>[4x]MGSSHHHHHHSGLVPRGSHMATPPKRSSPSFSASSEGTRIKKISIEGNIAAGKSTFVNILKQLSEDWEVVPEPVARWSNVQSTQDEFEELTMSQKNGGNVLQMMYEKPERWSFTFQTYACLSRIRAQLASLNGKLKDAE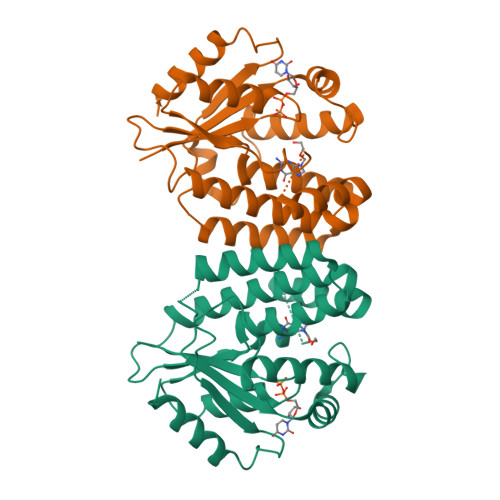KPVLFFERSVYSDRYIFASNLYESESMNETEWTIYQDWHDWMNNQFGQSLELDGIIYLQATPETCLHRIYLRGRNEEQGIPLEYLEKLHYKHESWLLHRTLKTNFDYLQEVPILTLDVNEDFKDKYESLVEKVKEFLSTL>MSNLPVEPEFEQAYKELASTL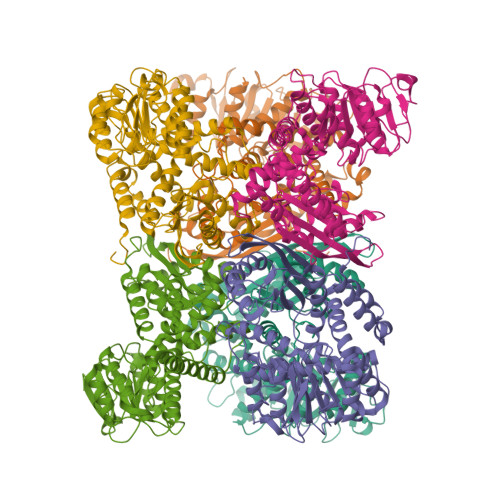ENSTLFQKNPEYRKALAVVSVPERVIQFRVVWENDKGEVQVNRGFRVQFNSALGPYKGGLRFHPSVNLSILKFLGFEQIFKNALTGLNMGGGKGGSDFDPKGKSDSEIRRFCVAFMTELCRHIGADTDVPAGDIGVTGREIGYLFGQYRKLRNSWEGVLTGKGGSWGGSLIRPEATGYGVVYYVEHMIAHATNGAESFAGKRVAISGSGNVAQYAALKVIELGGSVVSLSDSQGSLIVNGEGSFTPAEIDAIAALKVDRKQIAELVTDAAFADKFTYLPGQRPWVHVGAVDVALPSATQNEVSGEEAQALIAAGCKFIAEGSNMGCTQAAIDAFEAHREANKGAAAIWYAPGKAANAGGVAVSGLEMAQNSARLSWTAEEVDARLKDIMKSCFQNGLDTAKEYATPADGILPSLVTGSNIAGFTKVAAAMKDQGDWW[2x]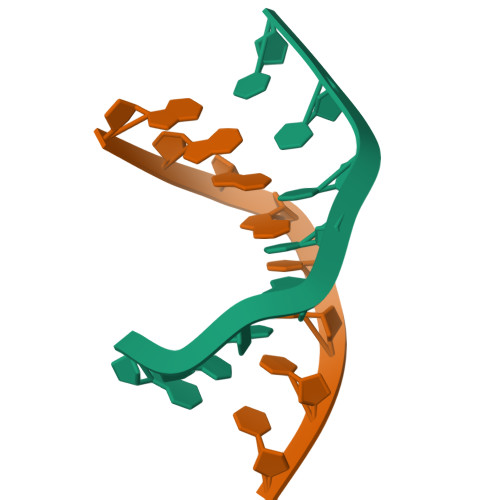>[4x]GAAGCTTC>MRGSHHHHHHGSMSSGNSSLGIIVGIDDSPAAQVAVRWAARDAELRKIPLTLVHAVSPEVATWLEVPLPPGVLRWQQDHGRHLIDDA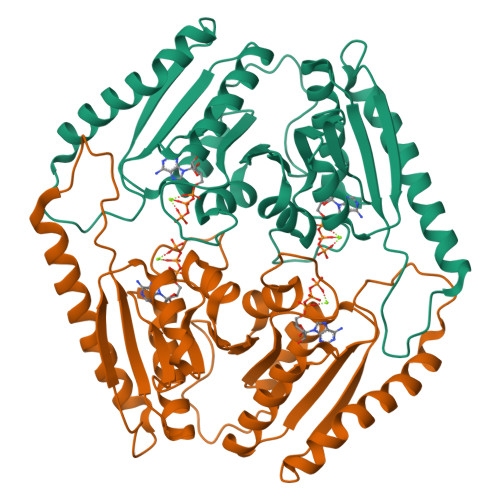LKVVEQASLRAGPPTVHSEIVPAAAVPTLVDMSKDAVLMVVGCLGSGRWPGRLLGSVSSGLLRHAHCPVVIIHDEDSVMPHPQQAPVLVGVDGSSASELATAIAFDEASRRNVDLVALHAWSDVDVSEWPGIDWPATQSMAEQVLAERLAGWQERYPNVAITRVVVRDQPARQLVQRSEEAQLVVVGSRGRGGYAGMLVGSVGETVAQLARTPVIVARESLT[8x]propan-2-yl {[4-ethoxy-3-(1-methyl-7-oxo-3-propyl-6,7-dihydro-1H-pyrazolo[4,3-d]pyrimidin-5-yl)phenyl]sulfonyl}carbamate 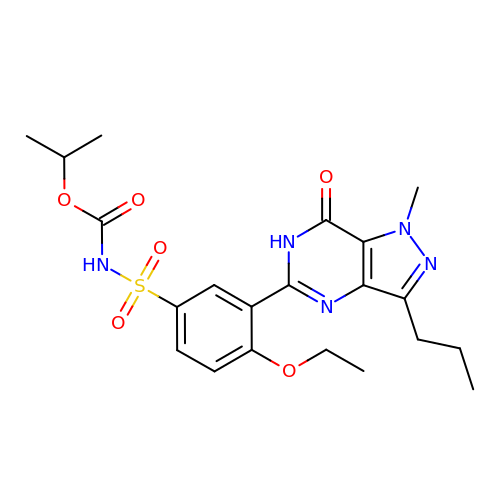| C21 H27 N5 O6 S | RGTRFWTZGHUUBF-UHFFFAOYSA-N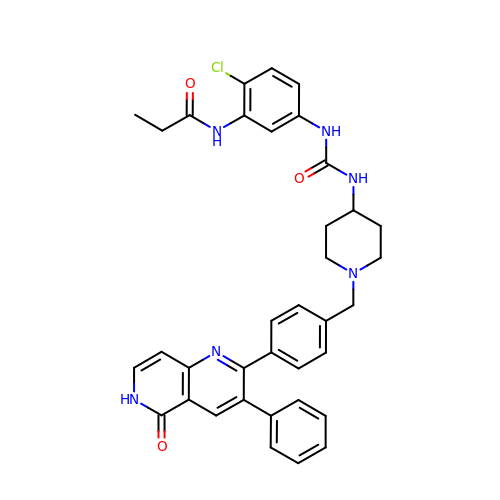~{N}-[2-chloranyl-5-[[1-[[4-(5-oxidanylidene-3-phenyl-6~{H}-1,6-naphthyridin-2-yl)phenyl]methyl]piperidin-4-yl]carbamoylamino]phenyl]propanamide | C36 H35 Cl N6 O3 | JIITZXKZXZZBIZ-UHFFFAOYSA-N> NGPSPNLPPGFDFTDPAIYAERLPVAEFAELRSAAPIWWNGQDPGKGGGFHDGGFWAITKLNDVKEISRHSDVFSSYENGVIPRFKNDIAREDIEVQRFVMLNMDAPHHTRLRKIISRGFTPRAVGRLHDELQERAQAIAAEAAAAGSGDFVEQVSCELPLQAIAGLLGVPQEDRGKLFHWSNEMTGNEDPEYAHIDPKASSAELIGYAMKMAEEKAKNPADDIVTQLIQADIDGEKLSDDEFGFFVVMLAVAGNETTRNSITQGMMAFAEHPDQWELYKKVRPETAADEIVRWATPVTAFQRTALRDYELSGVQIAAGQRVVMFYRSANFDEEVFQDPFTFNILRNPNPHVGFGGTGAHYCIGANLARMTINLIFNAVADHMPDLKPISAPERLRSGWLNGIKHWQVDYTGRCPVA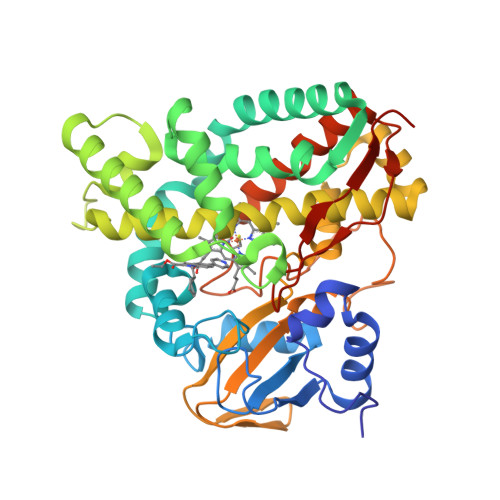H>MSGHHHHHHFRGRIELIIGPMFAGKTTELMRRVKREIHARRSCFVIKYSKDTRYDEHNVASHDQLMLRAQAAVSQLTEVRDTWKRFDVLAIDEGQFFSDLVDFCNTAADAGKVVMVSALDGDYRRKPFGQICELVPYCEAVDKLTAVCMMCHEQPACFTRRTVNVEQQELIGGADMYIATCRECY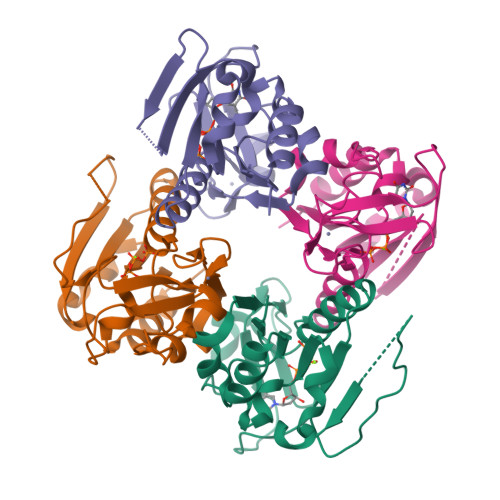SKQQLP[8x]>[2x]HHHHHHGSMAPKRSSDLFSQVVNSGPGSFLARQLGVPQPETLRRYR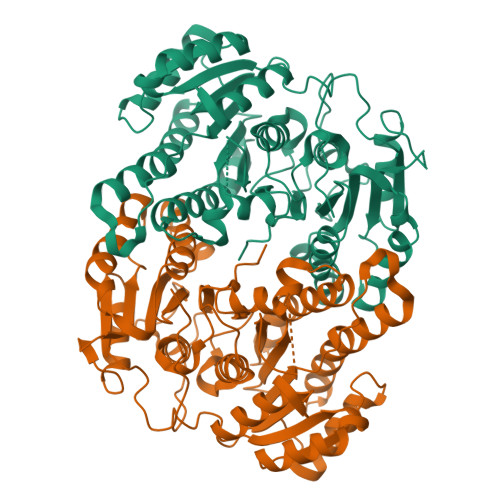AGEPPLTGSLLIGGAGRVVEPLRAALEKDYDLVGNNLGGRWADSFGGLVFDATGITEPAGLKGLHEFFTPVLRNLGRCGRVVVVGGTPEAAASTNERIAQRALEGFTRSLGKELRRGATTALVYLSPDAKPAATGLESTMRFLLSAKSAYVDGQVFSVGADDSTPPADWEKPLDGKVAIVTGAARGIGATIAEVFARDGAHVVAIDVESAAENLAETASKVGGTALWLDVTADDAVDKISEHLRDHHGGKADILVNNAGITRDKLLANMDDARWDAVLAVNLLAPLRLTEGLVGNGSIGEGGRVIGLSSIAGIAGNRGQTNYATTKAGMIGITQALAPGLAAKGITINAVAPGFIETQMTAAIPLATREVGRRLNSLLQGGQPVDVAEAIAYFASPASNAVTGNVIRVCGQAMIGA> DAAQPARRARRTYEAYPAKPKCPAVCTCTKDNALCENARSIPRTVPPDVISLSFVRSGFTEISEGSFLFTPSLQLLLFTSNSFDVISDDAFIGLPHLEYLFIENNNIKSISRHTFRGLKSLIHLSLANNNLQTLPKDIFKGLDSLTNVDLRGNSFNCDCKLKWLVEWLGHTNATVEDIYCEGPPEYKKRKINSLSSKDFDCIITEFAKSQDLPYQSLSIDTFSYLNDEYVVIAQPFTGKCIFLEWDHVEKTFRNYDNITGTSTVVCKPIVIETQLYVIVAQLFGGSHIYKRDSFANKFIKIQDIEILKIRKPNDIETFKIENNWYFVVADSSKAGFTTIYKWNGNGFYSHQSLHAWYRDTDVEYLEIVRTPQTLRTPHLILSSSSQRPVIYQWNKATQLFTNQTDIPNMEDVYAVKHFSVKGDVY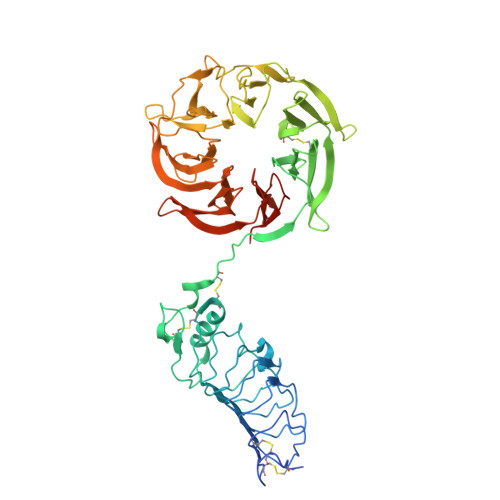ICLTRFIGDSKVMKWGGSSFQDIQAMPSRGSMVFQPLQINNYQYAILGSDYSFTQVYNWDAEKAKFVKFQELNVQAPRSFTHVSINKRNFLFASSFKGNTQIYKHVIVDLSAKHHHHHH> MLRSANPTIAKALQPLIEGPKFAVVYCGNHQYKVSPGDVIAVQRLRAPIGSQIALKKVLMVGGPRFTAIGRPLLEHVRVTADVEEQKRMRNVVSLFSTPGRRRLRWLDAQHAATILRIREVVYEPTVVGELDKYDGVLLKD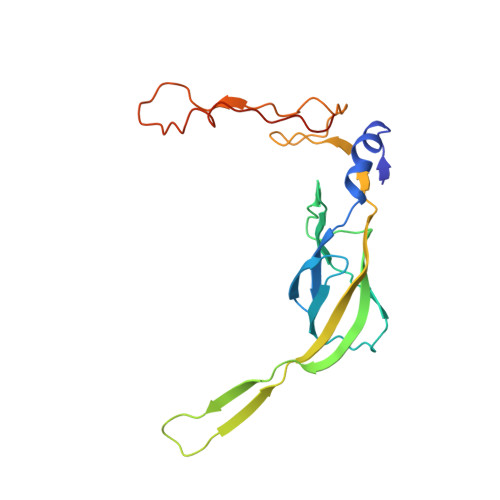FHADRHPNPVFTANDGYDLYYPKDWNKVEEASAFLEMMEAPPTEK> MTNIEPVIIETRLELIGRYLDHLKKFENISLDDYLSSFEQQLITERLLQLITQAAIDINDHILSKLKSGKSYTNFEAFIELGKYQILTPELAKQIAP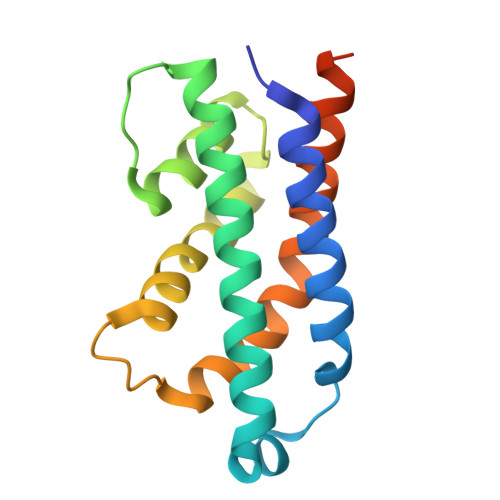SSGLRNRLVAEFDDIDPNQVFMAISFALQQYPLYVRQINSYLITLEEENDLESGHHHHHH> GPAAPAQSPAAPDPEASPLAEPPQEQSLAPWSPQTPAPPCSRCFARAIESSRDLLHRIKDEVGAPGIVVGVSVDGKEVWSEGLGYADVENRVPCKPETVMRIASISKSLTMVALAKLWEAGKLDLDIPVQHYVPEFPEKEYEGEKVSVTTRLLISHLSGIRHYEKDIKKVKEEKAYKALKMMKENVAFEQEKEGKSNEKNDFTKFKTEQENEAKCRNSKPGKKKNDFEQGELYLREKFENSIESLRLFKNDP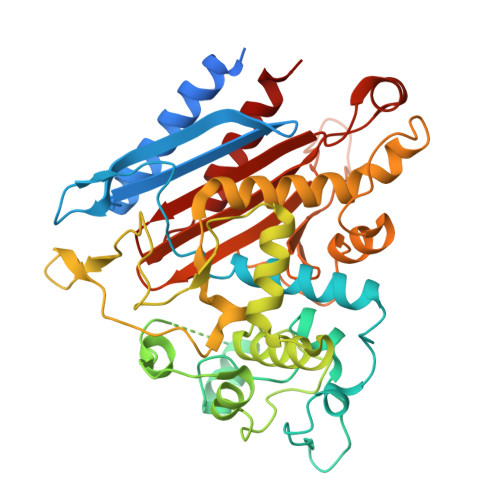LFFKPGSQFLYSTFGYTLLAAIVERASGCKYLDYMQKIFHDLDMLTTVQEENEPVIYNRARFYVYNKKKRLVNTPYVDNSYKWAGGGFLSTVGDLLKFGNAMLYGYQVGLFKNSNENLLPGYLKPETMVMMWTPVPNTEMSWDKEGKYAMAWGVVERKQTYGSCRKQRHYASHTGGAVGASSVLLVLPEELDTETINNKVPPRGIIVSIICNMQSVGLNSTALKIALEFDKDRSD>[2x]GS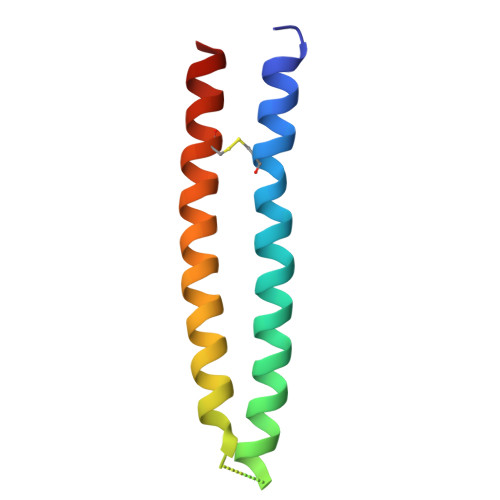MTISNMEADCNRLLKQREELTKRREKLSKRREKIVKENGEGDKNVANINEEMESLTANIDYINDSISDCQANIMQMEEAK N-(methoxycarbonyl)-beta-D-glucopyranosylamine | C8 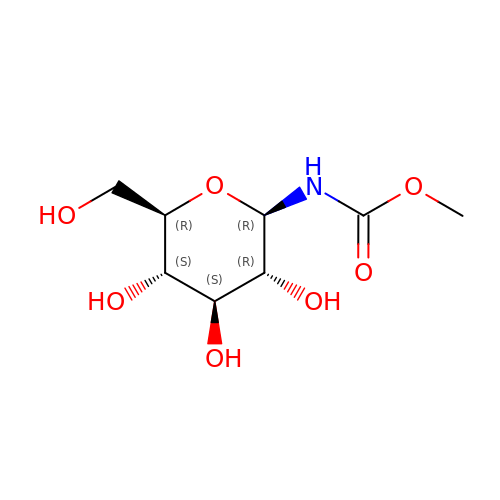H15 N O7 | IZZJOGWXTFEDLL-XUUWZHRGSA-N> GDQITKMKDRLVEWNDQVEKLGKKMEAR;> SQLLNEWSHNVDELLEHIETIGHLITKEEIMHGL;> ATYDSALELVGQLNKVVDQLFEKAS;> NAQYHLLVKQGDGLLTKLQKYGAAVR;> EDPQ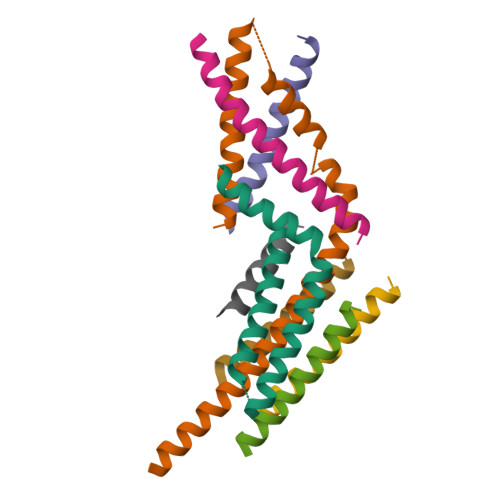QVFDERIKFANQLHDEYLVS;> KTNIIEKAMDYAISIEN;> IRLTNQLKSLKGLQSKLKDVVEYLDKVINKELPINHTILGKLQDVFNLLPNLGTPDDDEIDVENHDRINISNNLQKALTVKTNDELMVIYISNLVRSIIAFDDLIENKIQNKKIQEQRVKD;> YEEKEESNLAATKSMVKIAEQYSKRIEEEKELTEEELKTRYVGRQDPKKHLSETADETLENNIVSVLTA>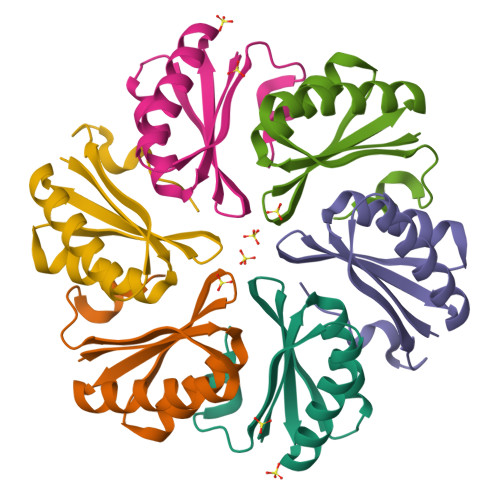[9x]MHHHHHHQQEALGMVETKGLTAAIEAADAMVASANVMLVGYEKIGQGLVTVIVRGDVGAVKAATDAGAAAARNVGEVKAVHVIPRPHTDVEKILPKGISQ> KETAAAKFERQHMDSSTSAASSSNYCNQMMKSRNLTKDRCKPVNTFVHESLADVQAVCSQKNVACKNGQTNCYQSYSTMSITDCRETGS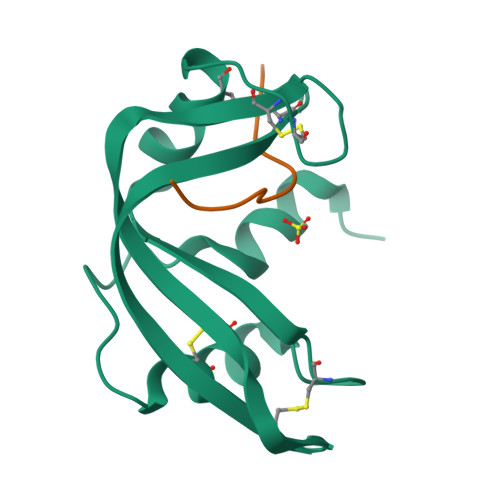SKYPNCAYKTTQANKHIIVACEGNPYVPV;> EGSPYVPVHYDASV>QAMTKTL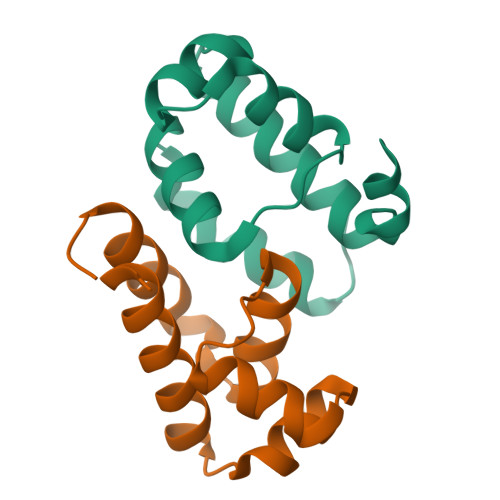RTPEHVYLCQRLRQARLDAGLTQADLAERLDKPQSFVAKVETRERRLDVIEFAKWMAACEGLDVVSEIVATIAEGRAQA[2x]>[9x]MDAEGLALLLPPVTLAALVDSWLREDCPGLNYAALVSGAGPSQAALWAKSPGVLAGQPFFDAIFTQLNCQVSWFLPEGSKLVPVARVAEVRGPAHCLLLGERVALNTLARCSGIASAAAAAVEAARGAGWTGHVAGTRKTTPGFRLVEKYGLLVGGAASHRYDLGGLVMVKDNHVVAAGGVEKAVRAARQAADFALKVEVECSSLQEAVQAAEAGADLVLLDNFKPEELHPTATVLKAQFPSVAVEASGGITLDNLPQFCGPHIDVISMGMLTQAAPALDFSLKLFAKEVAPVPKIHLEHHHHHH

QPRTs have been shown to exist as dimers or hexamers2223242526272829. HsQPRT is regulated by the interaction between two dimeric subunits. which can adopt open and closed states.

complex with QA or NAMN as a reactant or product. First, loops L and O of HsQPRT were closed upon QA binding. chain of H160 in addition to its interaction with the carboxylate moiety of QA. moiety of QA and tartrate molecules of 2.4 Å. relevance of HsQPRT-QA compared with tartrate as a QA mimic. can occupy the active site before PRPP enters. PRPP bound to the carboxylate moiety of QA to produce NAMN.> MGKSSKDKRDLYYRKAKEQGYRARSAFKLLQLNDQFHFLDDPNLKRVVDLCAAPGSWSQVLSRKLFDESPSSDKEDRKIVSVDLQPMSPIPHVTTLQADITHPKTLARILKLFGNEKADFVCSDGAPDVTGLHDLDEYVQQQLIMS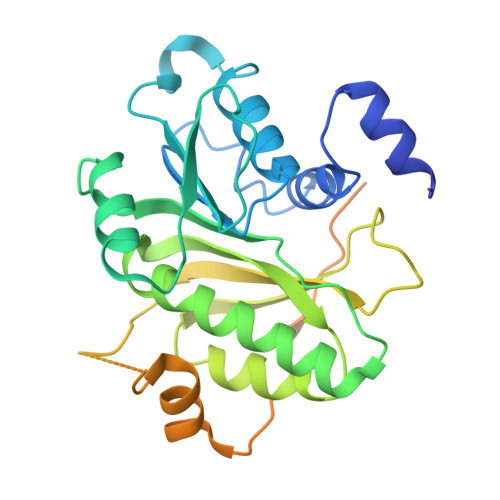ALQLTACILKKGGTFVAKIFRGRDIDMLYSQLGYLFDKIVCAKPRSSRGTSLEAFIVCLGYNPPSNWTPKLDVNTSVDEFFQGCFLNKLCISDKLSHWNEEERNIAEFMACGSLQSFDSDATYHDLPSSVAGTSSSLDPVQSPTNPPYKKALELKRSGKLTRSVLEVLFQGPSHHHHHH> TCNIKNGRCEQFCKNSADNKVVCSCTEGYRLAENQKSCEPAVPFPCGRVSVSQTSKLTR;> FPR;> VVGGEDAKPGQFPWQVVLNGKVDAFCGGSIVNEKWIVTAAHCVETGVKITVVAGEHNIEETEHTEQKRNVIRIIPHHNFNAAINTYNHDIALLELDEPLVLNSYVTPICIADKEYTNIFLKFGSGYVSGWGRVFHKGRSALVLQYLRVPLVDRATCLRSTKFTITNNMFCAGFHEGGRDSCQGDSGGPHVTEVEGTSFLTGIISWGEECAMKGKYGIYTKVSRYVNWIKEKTKL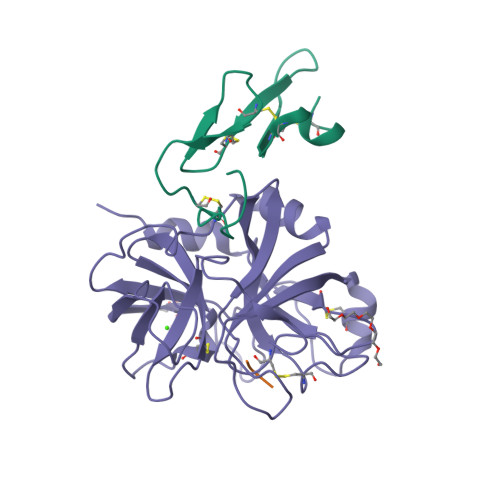T>[2x]MGSSHHHHHHSSGENLYFQGEAVVISGRKLAQQIKQEVRQEVEEWVASGNKRPHLSVI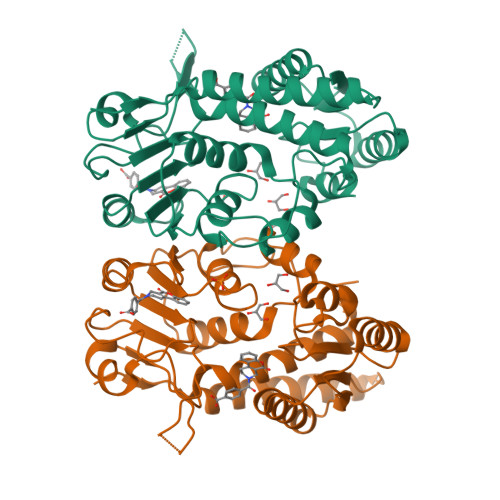LVGENPASHSYVLNKTRAAAVVGINSETIMKPASISEEELLNLINKLNNDDNVDGLLVQLPLPEHIDERRICNAVSPDKDVDGFHVINVGRMCLDQYSMLPATPWGVWEIIKRTGIPTLGKNVVVAGRSKNVGMPIAMLLHTDGAHERPGGDATVTISHRYTPKEQLKKHTILADIVISAAGIPNLITADMIKEGAAVIDVGINRVHDPVTAKPKLVGDVDFEGVRQKAGYITPVPGGVGPMTVAMLMKNTIIAAKKVLRLEERE> MAHHHHHHMISTAETGREPVYSLTGKKIFVAGHTGMVGSAILRRLQHEDCDIITAAHSVLDLTRQGPTENFISGHRPDVIIIAAARVGGILANSRFPADFLYDNLAIGMNLIHAAHQIGVERLLWLGSSCIYPRDAAQPLTEDALLTGPLEPTNEAYAIAKIAGLKYAQSCARQFGDRFITAMPTNLYGPNDNFDPTSSHVLPALIRRVHEAR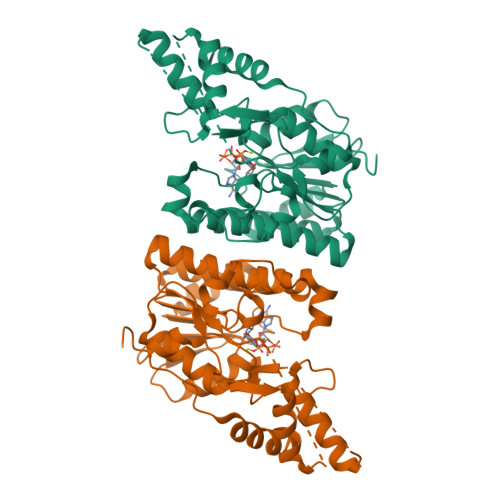MRGAEEVVLWGSGKPLREFLHVDDLADACLHLLRFYNGIEPVNIGSGEEISIKELALTVARIVGYEGRFEHDLSKPDGTPRKLLDTSRIEALGWQPRIRLEDGLRDVYRNWLEETAGSVAA> GTSSMADIGSRYSKISDNYSSLLQVSEALGRAGLESSNLIVGIDFTKSNEWTGAKSFNRKSLHHLSNTPNPYEQAITIIGRTLAAFDEDNLIPCYGFGDASTHDQDVFSFYPEGRFCNGFEEVLARYREIVPQLKLAGPTSFAPIIEMAMTVVEQSSGQYHVLVIIADGQVTRSVDTEHGRLSPQEQKTVDAIVKASTLPLSIVLVGVGDGPWDMMQEFDDNIPARAFDNFQFVNFTEIMSKNKDQSRKETEFALSALMAIPPQYKATIELNLLGVRNGNIPQRIPLPPPV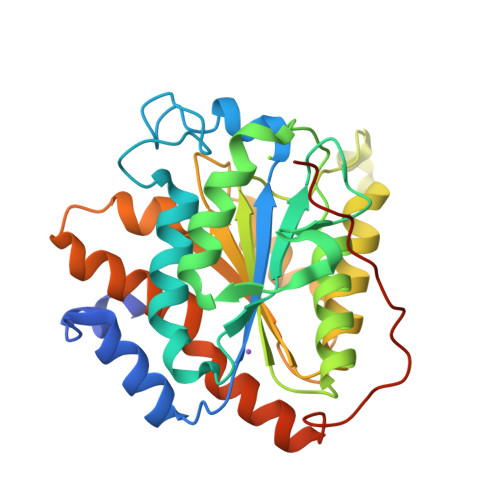QSGSSFSSSR>GSMAPLVKNEPQHAKILAIGTANPPNVYHQKDYPDFLFRVTKNEHRTDLREKFDRICEKSRTKKRYLHLTEEMLKANPNIYTYGAPSLDVRQDICNIEVPKLGQEAALKAIKEWGQPISRITHLIFCTASCVDMPGCDFQLIKLLGLDPSVTRTMIYEAGCYAGATVLRMAKDFAENNKGARVLVVCAEITTVFFHGL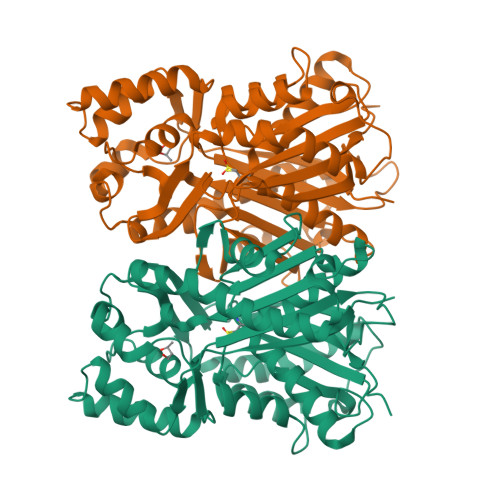TDTHLDILVGQALFADGASAVIVGANPEPEIERPLFEIVACRQTILPNSEHGVVANIREMGFNYYLSGDVPKFVGGNVVDFMTKTFEKVDGKKKDWNSLFFSVHPGGPAIVDQVEEKLGLKEGKLRATRHVLSEYGNMGAPTVHFILDEMRNKSIEEGKTTTGEGLEWGVVIGIGPGLTVETAVLRSESIRC[2x]>[2x]MHVFYSEERRGNLLILREGEVKHFRVRRIEKDEEFGVIHEGKIYVCKVRREDKREISCEIVEELETKLPPKDITLYQSVTVDLKTMDTI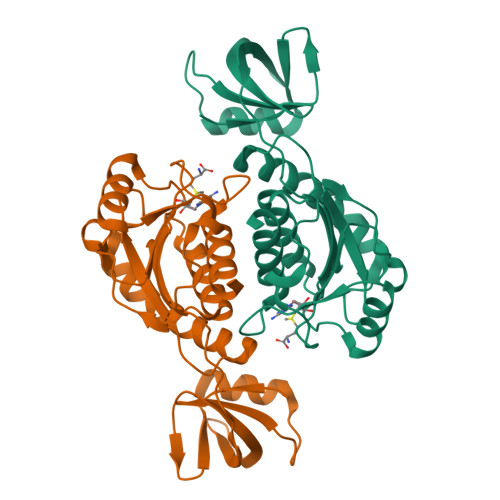VRQATELGVLTFVPIISERSFQKEEAILKKTEKWKRIVIEAMKQSRRPIPMEIKKPVRLSDLIPESEENIILDNFYEGVKPKDVNLEAKTYSVVVGPEGGFSKRESQILREKGFKSVLLEPYTLRTETAVVSIVSILMNF> MGFL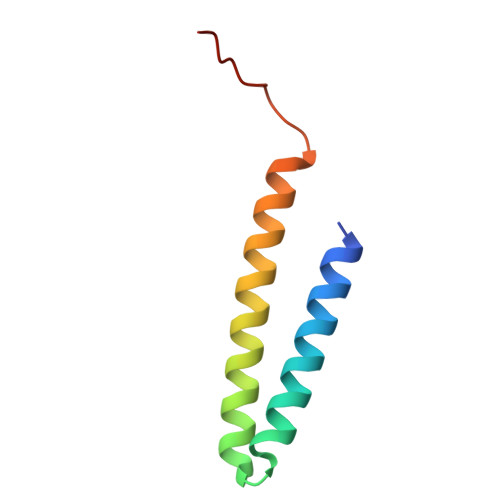VTTLVFLVIGIIASLCTRICCNRGPSTNLLHLTLVITATVSCWMMWAIVYLAQMKPLIVPILSEEE> MTVTTTYPGVYLSEDAVSSFSVNSAATAVPLFAYDSENTNTINKPIQVFRNWAEFTVEYPTPLEDAFYTSLSLWFMHGGGKCYLVNEANIADAVAQYDDITLIVAAGTDTTTYTAFTTVVGQGYRIFGLFDGPKEKIAGTAKPDEVMEEYPTSPFGAVFYPWGTLASGAAVPPSAIAAASITQTDRTRGVW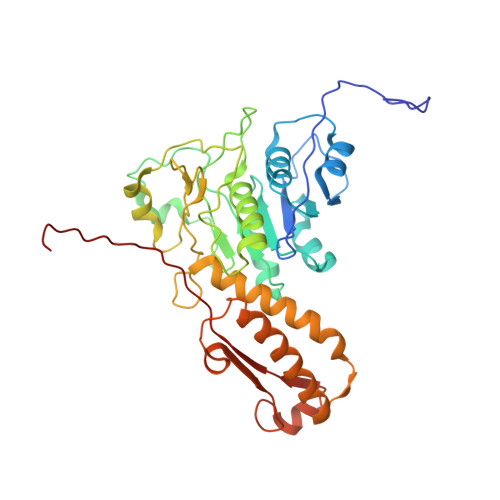KAPANQAVNGVTPAFAVSDDFQGKYNQGKALNMIRTFSGQGTVVWGARTLEDSDNWRYIPVRRLFNAVERDIQKSLNKLVFEPNSQPTWQRVKAAVDSYLHSLWQQGALAGNTPADAWFVQVGKDLTMTQEEINQGKMIIKIGLAAVRPAEFIILQFSQDIAQ> TEFKAGSAKKGATLFKTRCLQCHTVEKGGPHKVGPNLHGIFGRHSGQAEG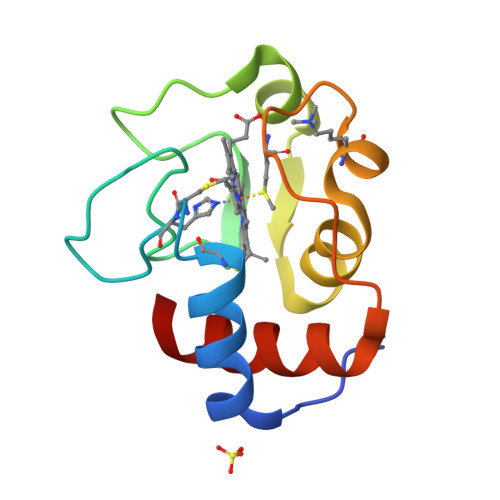YSYTDAIIKKNVLWDENNMSEFLTNPKKYIPGTKMAFGGLKKEKDRNDLITYLKKATE>MSAELASRGRKVYFVGLNEYPFLPLVAGLLRTYAEQDERIAAAYDFQEPVFLVAPVQEMADGIVEPDVLALSCYVWNFRRQMKVAKLVKERYPNVLVVAGGPHVPDRPGNFFEKHPYVDVLAHGEGEVAFRELLATRLSDHPDYTAVPGVSVRRGTEAVVGPKAKRLPRLIDTPSPYLLGVMDGAVATCRERGLRFYALWETNRGCPYSCSFCDWGSATMSTLRKFEDERLQDEIEWFARHDVEDLFICDANFGIMPRDLEIAHALAEARGELGAPRQVRVNFAKNSNDRVFDISKTWHDADLLMGTTLSMQSTDMDVLEAIDRKNIGLDNYRKLQQRYAAENIHTYTELILGLPMETARSFRDGIGSLLEAGNHEDLRVYELGILPNAPLNTPEKIEQYGLRTVPKRMYVERPGTPDDEAETFEMVMETNAMPRDAWVESFSFIQAVQFLHNGCYTRYLSIFLRQEHGIGYTRFYEGLQDYFTGRPDTVLGALYLRMRSLYHDYIDMPALPLANLVASQPDMAADLAPYGRRRGWTIDNWGWLRIATDFDRFHTELREYLATLGLDPAGDARLEDVLRFQQDVMLRPDYSPELGKSAEYAHDWPGYFAGGLLRPRR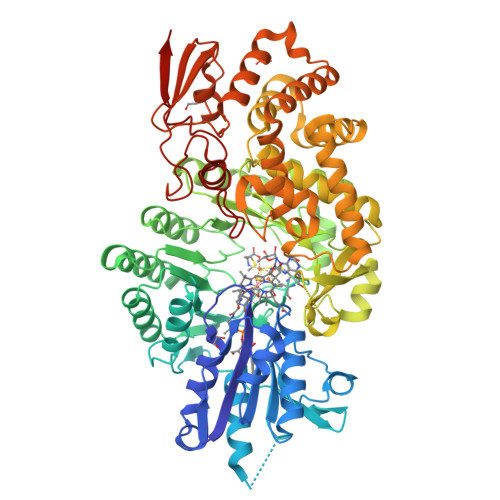VRVAYGDQSFGANGRYRPVPGDLKAFTMAAIGTSYPVSRMGHFCHRFESAEVTSLAEPVVSEQW[2x]> MSERIVISPTSRQEGHAELVMEVDDEGIVTKGRYFSITPVRGLEKMVTGKAPETAPVMVQRICGVCPIPHTLASVEAIDDSLDIEVPKAGRLLRELTLAAHHVNSHAIHHFLIAPDFVPENLMADAINSVSEIRKNAQYVVDMVAGEGIHPSDVRIGGMADNITELARKRLYARLKQLKPKVNEHVELMIGLIEDKGLPEGLGVHNQPTLASHQIYGDRTKFDLDRFTEIMPESWYDDPEIAKRACSTIPLYDGRNVEVGPRARMVEFQGFKERGVVAQHVARALEMKTALSRAIEILDELDTSAPVRADFDERGTGKLGIGAIEAPRGLDVHMAKVENGKIQFYSALVPTTWNIPTMGPATEGFHHEYGPHVIRAYDPCLSCATH;> MSLIARIKRFLGLEAEAKREEPEKEKSEPVGASKEEVEKVAEENAKPRIGYIHLSGCTGDAMSLTENYDILAELLTNMVDIVYGQTLVDLWEMPEMDLALVEGSVCLQDEHSLHELKELREKAKLVCAFGSCAATGCFTRYSRGGQQAQPSHESFVPIADLIDVDLALPGCPPSPEIIAKTVVALLNNDMDYLQPMLDLAGYTEACGCDLQTKVVNQGLCIGCGTCAMACQTRALDMTNGRPELNSDRCIKCGICYVQCPRSWWPEEQIKKELGL;> MVLGTYKEIVSARSTDREIQKLAQDGGIVTGLLAYALDEGIIEGAVVAGPGEEFWKPQPMVAMSSDELKAAAGTKYTFSPNVMMLKKAVRQYGIEKLGTVAIPCQTMGIRKMQTYPFGVRFLADKIKLLVGIYCMENFPYTSLQTFICEKLGVSMELVEKMDIGKGKFWVYTQDDVLTLPLKETHGYEQAGCKICKDYVAELADVSTGSVGSPDGWSTVITRTDAGDSIFKQAVEAGLFETKPIEEVKPGLGLLEKLAAQKKEKAEKNIAARKEMGLPTPF

Frh is a key enzyme in the metabolism of methanogenic archaea, where the reduction of carbon dioxide to methane involves the oxidation of four molecules of H2 by a number of different hydrogenases. Frh is a heterotrimeric enzyme composed of the 43 kDa subunit FrhA that contains a [NiFe]-center, the 26 kDa subunit FrhG with three [4Fe4S] clusters, and the 31 kDa iron–sulphur flavoprotein FrhB, which contains the F420-binding site and has one [4Fe4S] cluster and an FAD. Our cryo-EM study showed that the Frh complex is a dodecamer with tetrahedral symmetry. Electrons are extracted from hydrogen by the [NiFe] cluster in FrhA, and transferred via the three [4Fe4S] clusters in FrhG and another one in FrhB to FAD and from there to the substrate.

Refinement of this smaller dataset under otherwise identical conditions resulted in maps with better resolution than the full dataset, and the best map, with 6 frames averaged, extended to 3.36 Å resolution. All three subunits were traced completely except for a few N- or C-terminal residues, accounting for 893 out of 903 amino acids. In the new map, two nearby density features, modelled as extended loops before, were clearly recognizable as alpha-helices (194–201 and 208–215) that accommodate the missing residues. The resulting shift of residues brings the cysteine residues C206 and C208, which are conserved in the FrhG family, near a strong density on the dimer axis between two FrhG subunits. The cysteines of the dimer partner are just a few Å away, and the density in between the four cysteine side chains is strongly suggestive of a coordinated ion. The function of this ion is most likely to stabilize the dodecameric complex, but its location between the two medial FeS clusters at a distance of only 9 Å, which is less than the distance of ∼10 Å between adjacent FeS clusters in the electron transfer chains, means that a role in electron transfer cannot be ruled out. In the Falcon II map, the clusters are not just featureless blobs, but their tetrahedral coordination (mostly by cysteine residues, or, in one case, an aspartate) can be clearly seen. The FAD cofactor in FrhB has continuous density in the map, and its folded conformation with the adenine and isoalloxazine moieties in close proximity is confirmed. For the new Falcon-II map, we used an Frh sample with a large excess of F420, but the F420 binding pocket is clearly empty.> MSTPARRRLMRDFKRLQEDPPVGVSGAPSENNIMQWNAVIFGPEGTPFEDGTFKLVIEFSEEYPNKPPTVRFLSKMFHPNVYADGSICLDILQNRWSPTYDVSSILTSIQSLLDEPNPNSPANSQAAQLYQENKREYEKRVSAIVEQ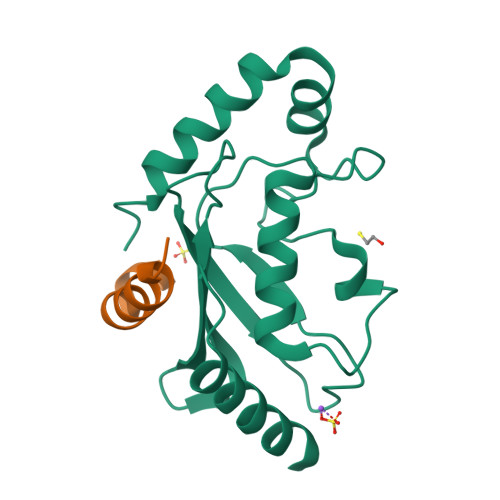SWNDS;> SKYRKKHKSEFQLLVDQARKGYKKIAG>[8x]GPLGSPSTDSLIKVDMRTISFDIPPQEVLTKDSVTISVDGVVYYRVQNATLAVANITNADSATRLLAQTTLRNALGTKNLSQILSDREEIAHHMQSTLDDATD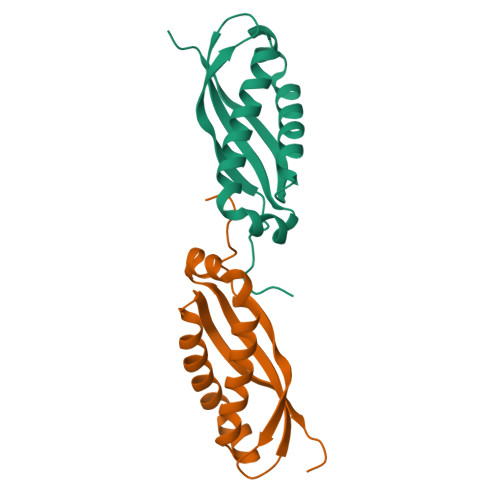DWGIKVERVEIKDVKLPVQLQRAMAAEAEA>MTDPNSPYFEKVLGSLFARQVEPAKDYAWDMGSTLPTPDDLMRRFIVKDTLITIFRRHGAVEAPTATLYPKSSHYGPNAVHLLDRNGTVLQLPCDLVMGHARSLARIASGPVPQRAYSFGNIFRDRQDGGQPDVYGEVDFDIVTTDAMDLAMKEAEVIKVLDEIIAAFPTTSSTPMCFQLGHSDLLQLIFDFCNVEHGARQAAAEVLSKLNIRNFTWQKVRSELRSPLVGISATSVDELQRFDWRDTPTKAFTKIRNLFEGTEYYDKVSSTLAHLKEVYEYSKKFKVNTKIYIAPLSSINEAFFRGGILFSCLYDRKVMDVFAAGGRYDSLIKAHRPRIGSRFEERHAVGFSLNWEKQLAKPVPKTTGKAFLKKAAEEEAQGIFSAKRCDVLVASFDPSILRSSGIELLQMLWAHGISAELARDARSPEDLLTTYRDESYSWIVIIKQESQLKIKTMHRKDVPDA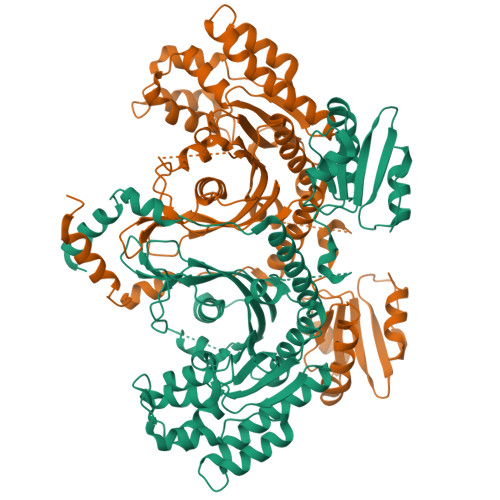DIQAKDLLAWLKAEI[2x]>MSGEHPSIDRDPYVVD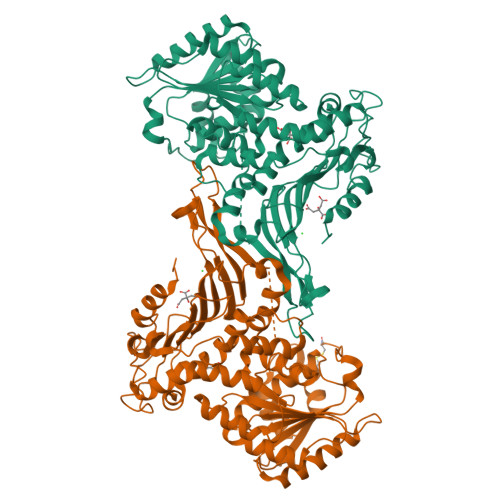LDTILDNLREQVLDKKPDDVLKFISKSALTLQSDEKRESCERIVSKVSEEQKRRPLTVVVLGASGDLAKKKTFPALFQLYCDGLLPPQINIVGYARTKQDDVEKWKHETLTKYFSRLHERSCHVEPFLKHVTYFTGSYDKKEDFQRLDEHVSKLEDAFDGEEKAGDRLFYLALPPSAFAGACGSIRAGAMPREGGWIRVIIEKPFGHDTESSAELSKAIEPFFDESQIYRIDHYLGKEMVQNIITTRFANRIFSALWNSNNIACVQITFKETIGTEGRGGYFDSIGIIRDVMQNHLTQILALLAMEKPNSLDAERIRDEKVSLLKCIAPIGKDDCVLGQYTASADGSIPGYLEDETVPKGSTCPTFAVLRLHINNDRWAGVPFILKAGKAVEQKYVAIRIQFKDEIRPYGDAAQRNELVIRAQPSEAMYMKITTKMPGLNEDLRETHQTELDLTYHSRFNVHLPDAYESLISDALRGNSTNFVRKDELDVAWRIFTPLLHQIDKGEVKPIPYQAGTRGPKEADDFILNSGFKFQKGYHWLAPNKLGHHHHHH[2x]>GSHMPKKKIQLHAE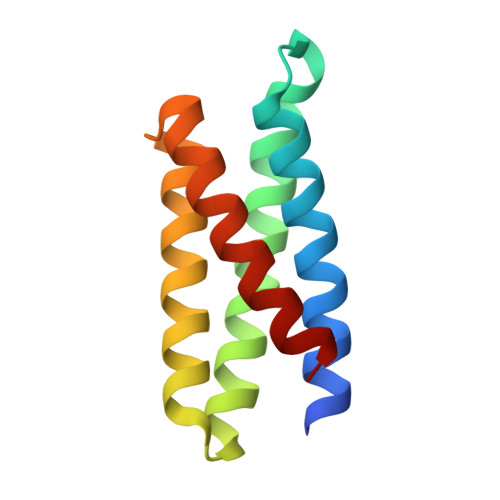HALYDALMILNIVKTNSPPAEEKLEDYAFNFELILEEIARLFESGDQKDEAEKAKRMKEWMKRIKTTASEDEQEEMANAIITILQSWIFS[6x]bufalin | C24 H34 O4 | 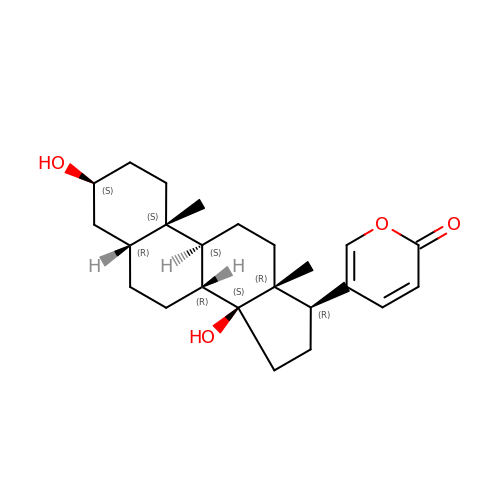QEEBRPGZBVVINN-BMPKRDENSA-N> TTGHSYEKYNNWETIEAWTKQVTSENPDLISRTAIGTTFLGNNIYLLKVGKPGPNKPAIFMDCGFHAREWISHAFCQWFVREAVLTYGYESHMTEFLNKLDFYVLPVLNIDGYIYTWTKNRMWRKTRSTNAGTTCIGTDPNRNFDAGWCTTGASTDPCDETYCGSAAESEKETKALADFIRNNLSSIKAYLTIHSYSQMILYPYSYDYKLPENNAELNNLAKAAVKELATLYGTKYTYGPGATTIYPAAGGSDDWAYDQGIKYSFTFELRDKGRYGFILPESQ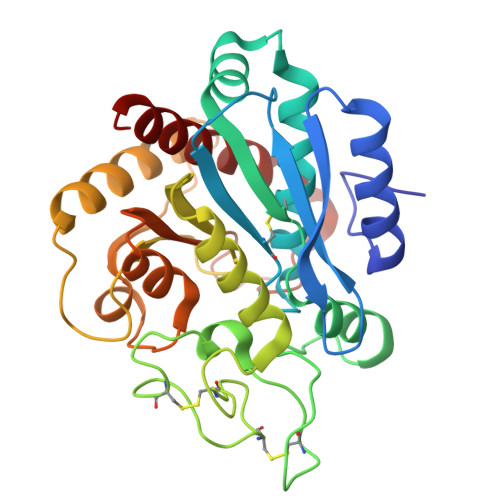IQATCEETMLAIKYVTNYVLGHL>[4x]MSKLQDVIVQEMKVKKRIDSAEEIMELKQFIKNYVQSHSFIKSLVLGISGGQDSTLVGKLVQMSVNELREEGIDCTFIAVKLPYGVQKDADEVEQALRFIEPDEIVTVNIKPAVDQSVQSLKEAGIVLTDFQKGNEKARERMKVQFSIASNRQGIVVGTDHSAENITGFYTKYGDGAADIAPIFGLNKRQGRQLLAYLGAPKELYEKTPTADLEDDKPQLPDEDALGVTYEAIDNYLEGKPVTP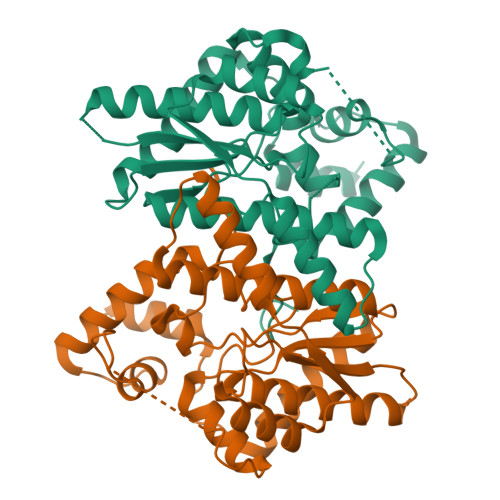EEQKVIENHYIRNAHKRELAYTRYTWPKSLEHHHHHH> MKPEVEQELAHILLTELLAYQFASPVRWIETQDVFLKDFNTERVVEIGPSPTLAGMAQRTLKNKYESYDAALSLHREILCYSKDAKEIYYTPDPSELAAKEEPAKEEAPAPTPAANAPAPAAAAPAPVAAAAPAAAAAEIADEPVKASLLLHVLVAHKLKKSLDSIPMSKTIKDLVGGKSTVQNEILGDLGKEFGTTPEKPEETPLEELAETFQDTFSGALGKQSSSLLSRLISSKMPGGFTITVARKYLQTRWGLPSGRQDGVLLVALSNEPAARLGSEADAKAFLDSMAQKYASIVGVDLSSAASASGAAGAGAAAGAAMIDAGALEEITKDHKVLARQQLQVLARYLKMDLDNGERKFLKEKDTVAELQAQLDYLNAELGEFFVNGVATSFSRKKARTFDSSWNWAKQSLLSLYFEIIHGVLKNVDREVVSEAINIMNRSNDALIKFMEYHISNTDETKGENYQLVKTLGEQLIENCKQVLDVDPVYKDVAKPTGPKTAIDKNGNITYSEEPREKVRKLSQYVQEMALGGPITKESQPTIEEDLTRVYKAISAQADKQDISSSTRVEFEKLYSDLMKFLESSKEIDPSQTTQLAGMDVEDALDKDSTKEVASLPNKSTISKTVSSTIPRETIPFLHLRKKTPAGDWKYDRQLSSLFLDGLEKAAFNGVTFKDKYVLITGAGKGSIGAEVLQGLLQGGAKVVVTTSRFSKQVTDYYQSIYAKYGAKGSTLIVVPFNQGSKQDVEALIEFIYDTEKNGGLGWDLDAIIPFAAIPEQGIELEHIDSKSEFAHRIMLTNILRMMGCVKKQKSARGIETRPAQVILPMSPNHGTFGGDGMYSESKLSLETLFNRWHSESWANQLTVCGAIIGWTRGTGLMSANNIIAEGIEKMGVRTFSQKEMAFNLLGLLTPEVVELCQKSPVMADLNGGLQFVPELKEFTAKLRKELVETSEVRKAVSIETALEHKVVNGNSADAAYAQVEIQPRANIQLDFPELKPYKQVKQIAPAELEGLLDLERVIVVTGFAEVGPWGSARTRWEMEAFGEFSLEGCVEMAWIMGFISYHNGNLKGRPYTGWVDSKTKEPVDDKDVKAKYETSILEHSGIRLIEPELFNGYNPEKKEMIQEVIVEEDLEPFEASKETAEQFKHQHGDKVDIFEIPETGEYSVKLLKGATLYIPKALRFDRLVAGQIPTGWNAKTYGISDDIISQVDPITLFVLVSVVEAFIASGITDPYEMYKYVHVSEVGNCSGSGMGGVSALRGMFKDRFKDEPVQNDILQESFINTMSAWVNMLLISSSGPIKTPVGACATSVESVDIGVETILSGKARICIVGGYDDFQEEGSFEFGNMKATSNTLEEFEHGRTPAEMSRPATTTRNGFMEAQGAGIQIIMQADLALKMGVPIYGIVAMAATATDKIGRSVPAPGKGILTTAREHHSSVKYASPNLNMKYRKRQLVTREAQIKDWVENELEALKLEAEEIPSEDQNEFLLERTREIHNEAESQLRAAQQQWGNDFYKRDPRIAPLRGALATYGLTIDDLGVASFHGTSTKANDKNESATINEMMKHLGRSEGNPVIGVFQ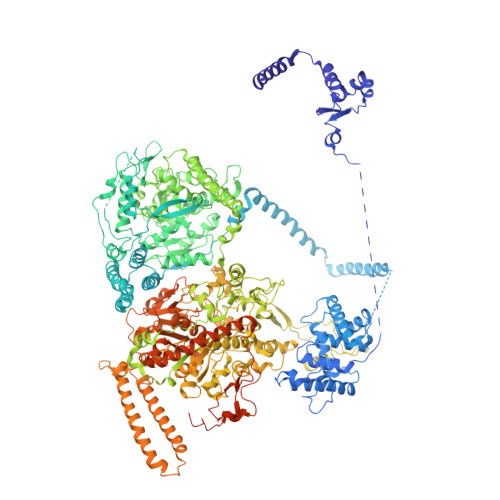KFLTGHPKGAAGAWMMNGALQILNSGIIPGNRNADNVDKILEQFEYVLYPSKTLKTDGVRAVSITSFGFGQKGGQAIVVHPDYLYGAITEDRYNEYVAKVSAREKSAYKFFHNGMIYNKLFVSKEHAPYTDELEEDVYLDPLARVSKDKKSGSLTFNSKNIQSKDSYINANTIETAKMIENMTKEKVSNGGVGVDVELITSINVENDTFIERNFTPQEIEYCSAQPSVQSSFAGTWSAKEAVFKSLGVKSLGGGAALKDIEIVRVNKNAPAVELHGNAKKAAEEAGVTDVKVSISHDDLQAVAVAVSTKK>[3x]MHHHHHHMKFLKPKINSFYAFEVKDAK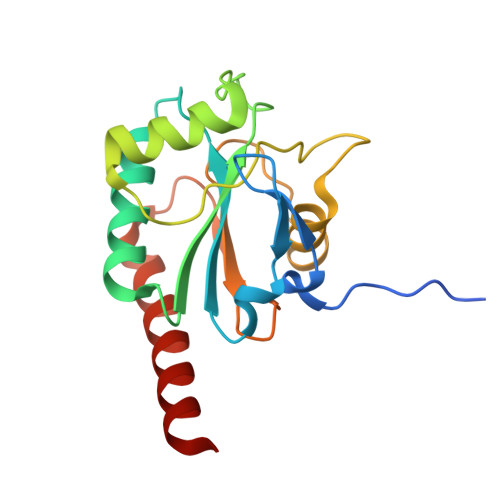GRTVSLEKYKGKVSLVVNVASDCQLTDRNYLGLKELHKEFGPSHFSVLAFPCNQFGESEPRPSKEVESFARKNYGVTFPIFHKIKILGSEGEPAFRFLVDSSKKEPRWNFWKYLVNPEGQVVKFWRPEEPIEVIRPDIAALVRQVIIKKKEDL>EFYHLVDDYGRGNGFFDKFNFFTGDDPTHGYVDYVSRDVAAGAGLIGERDGRTYMGVDFTNPASGRGRRSVRLESKNTYEHGLIVIDLAHMPGSVCGTWPAFWTLGTGDWPYGGEIDIIEGVNDNTFNHMVLHTSDGCTIDNDGFTGNLKTSNCYVYAPGQDANAGCGIEATDPNSYGKGFNSIGGGIYATEITPNGISIWFFPRGSEPGDVLGDNPNPANWDTPAAKFAGGGCDWEGKFNAQRLIFDVTFCGDWAGNVWGIGGCASRA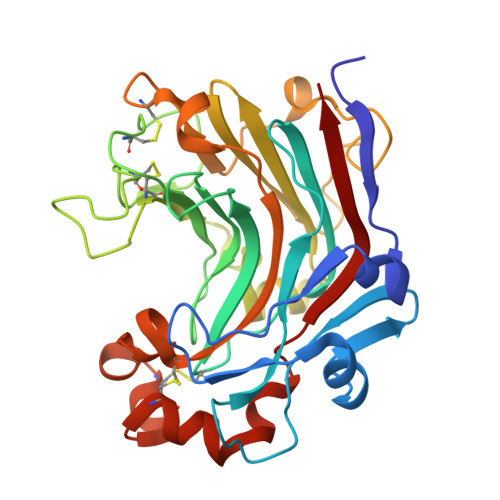ANCVDFVRDNPSAFAESYWLVNSLRVYAP[4x]>[2x]MRERLKRDLFQFNKTVEHGFPHQPSALGYSPSLRILAIGTRSGAIKLYGAPGVEFMGLHQENNAVTQIHLLPGQCQLVTLLDDNSLHLWSLKVKGGASELQEDESFTLRGPPGAAPSATQITVVLPHSSCELLYLGTESGNVFVVQLPAFRALEDRTISSDAVLQRLPEEARHRRVFEMVEALQEHPRDPNQILIGYSRGLVVIWDLQGSRVLYHFLSSQQLENIWWQRDGRLLVSCHSDGSYCQWPVSSEAQQPEPLRSLVPYGPFPCKAITRILWLTTRQGLPFTIFQGGMPRASYGDRHCISVIHDGQQTAFDFTSRVIGFTVLTEADPAAT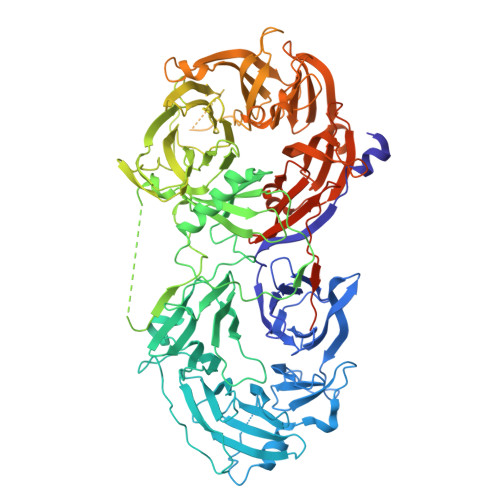FDDPYALVVLAEEELVVIDLQTAGWPPVQLPYLASLHCSAITCSHHVSNIPLKLWERIIAAGSRQNAHFSTMEWPIDGGTSLTPAPPQRDLLLTGHEDGTVRFWDASGVCLRLLYKLSTVRVFLTDTDPNENFSAQGEDEWPPLRKVGSFDPYSDDPRLGIQKIFLCKYSGYLAVAGTAGQVLVLELNDEAAEQAVEQVEADLLQDQEGYRWKGHERLAARSGPVRFEPGFQPFVLVQCQPPAVVTSLALHSEWRLVAFGTSHGFGLFDHQQRRQVFVKCTLHPSDQLALEGPLSRVKSLKKSLRQSFRRMRRSRVSSRKRHPAGPPGEAQEGSAKAERPGLQNMELAPVQRKIEARSAEDSFTGFVRTLYFADTYLKDSSRHCPSLWAGTNGGTIYAFSLRVPPAERRMDEPVRAEQAKEIQLMHRAPVVGILVLDGHSVPLPEPLEVAHDLSKSPDMQGSHQLLVVSEEQFKVFTLPKVSAKLKLKLTALEGSRVRRVSVAHFGSRRAEDYGEHHLAVLTNLGDIQVVSLPLLKPQVRYSCIRREDVSGIASCVFTKYGQGFYLISPSEFERFSLSTKWLVEPRCLVDSAETKNHRPGNGAGPKKAPSRARNSGTQSDGEEKQPGLVMEREFTTASENLYFQ> SNAMADE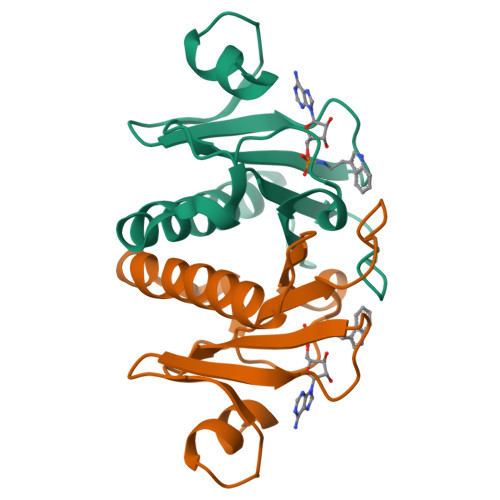IAKAQVARPGGDTIFGKIIRKEIPAKIIFEDDRCLAFHDISPQAPTHFLVIPKKHISQISVAEDDDESLLGHLMIVGKKCAADLGLNKGYRMVVNEGSDGGQSVYHVNLHVLGGRQMHWPPG>[4x]SIDQSVVISEKFANSIFAAVEHIKKQIKER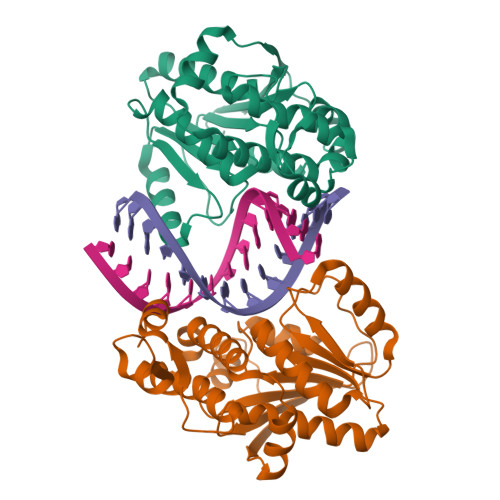DSNYKAIIFAPTVKFTSFLCSILKNEFKKDLPILEFHGKITQNKRTSLVKRFKKDESGILVCTDVGARGMDFPNVHEVLQIGVPSELANYIHRIGRTARSGKEGSSVLFICKDELPFVRELEDAKNIVIAKQEKYEPSEEIKSEVLEAVTEEPEDISDIVISLISSYRSCIKEYRFSERRILPEIASTYGVLLNDPQLKIPVSRRFLDKLGLSRSPIGKAMFEIRDY> SGFVCNTCPEKWINFQRKCYYFGKGTKQWVHARYACDDMEGQLVSIHSPEEQDFLTKHASHTGSWIGLRNLDLKGEFIWVDGSHVDYSNWAPGEPTSRSQGEDCVMM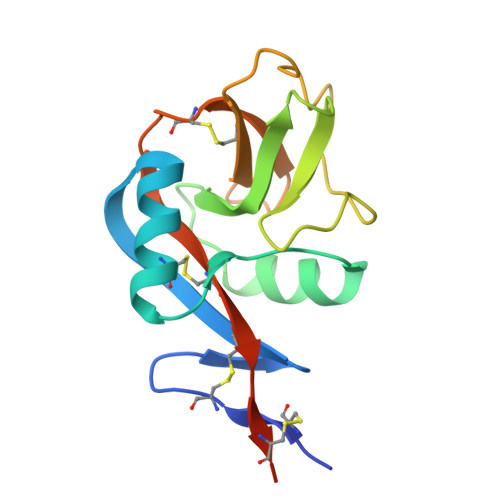RGSGRWNDAFCDRKLGAWVCDRLATCTPPASEGSAE> REATWVTEKPLTLKIHMHFRDKWVWDENWPVAREVARLTNVKLVGVANRAATNSQEQFNLMMASGQLPDIVGGDNLKDKFIRYGMEGAFIPLNKLIDQNAPNLKAFFKTHPEVQRAITAPDGNIYYLPYVPDGLVSRGYFIRQDWLDKLHLKTPQTVDELYTVLKAFKEKDPNGNGK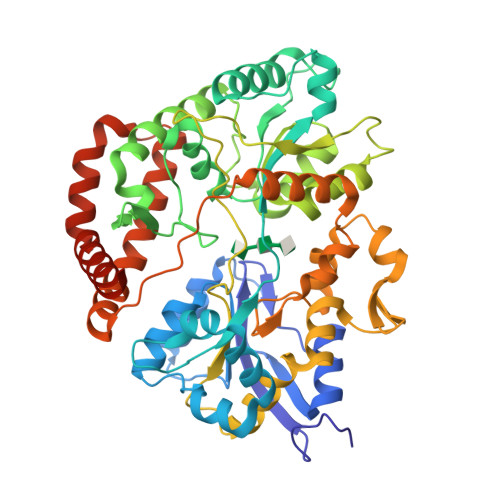ADEIPFINRDPEEVFRLVNFWGARSTGSNTWMDFYVENGKIKHPFAEVAFKDGIKHVAQWYKEGLIDPEIFTRKARSREQTFGNNIGGMTHDWFASTALFNDALSKNIPGFKLVPMAPPINSKGQRWEEDARQIPRPDGWAITATNKNPVETIKLFDFYFGPKGRELSNFGVPGLTYDIKNGKPVYKDTVLKAAQPVNNQMYDIGAQIPIGFWQDYEYERQWTNDVALQGIDMYIKNKYVLPQFTGVNLTVEEREIYDKYWPDVKTYMFEMGQSWVMGTKDPEKTWNDYQQQLKNRGFYQVMIVMQKAYDRQYGGAAKPAQVGAK6-(3-fluorophenyl)-N-[1-(2,2,2-trifluoroethyl)piperidin-4-yl]pyridine-3-carboxamide 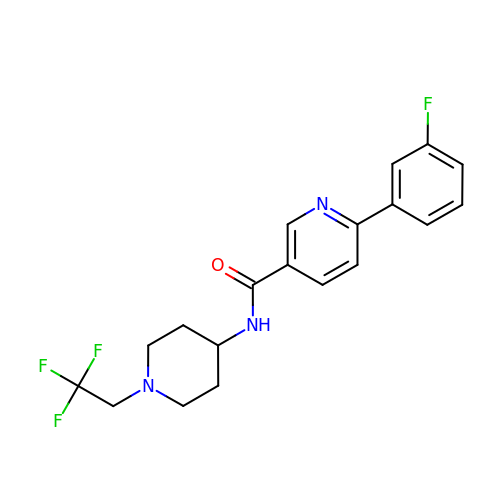| C19 H19 F4 N3 O | LPUCBGGXXIUBAZ-UHFFFAOYSA-N> ARARKGALVQCDPSIKALILQIDAKMSDIVLEELDDTHLLVNPSKVEFVKHELNRLLSKNIY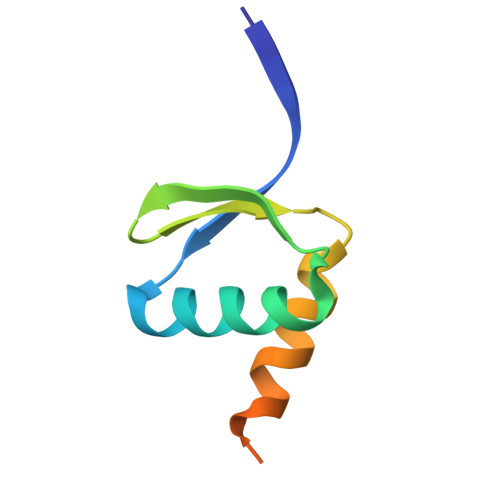NPMDEEENQ>ESEKIYKVMEEIFVDRHYKENIRTGEEVKQYFSKSKAEFILRWSSANESDTENKYVFIAASFQASDGIHSIR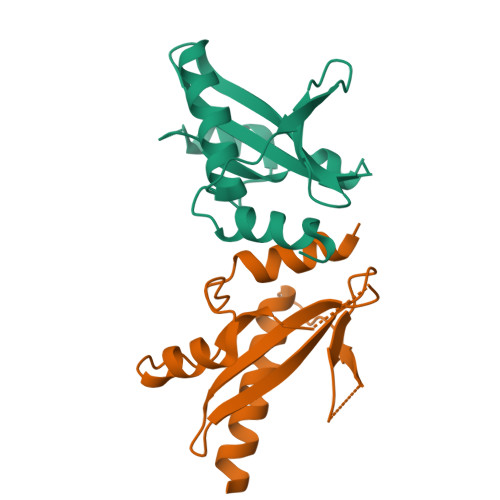YGINKNGELFSINTASNKVTPIDILPLGVMATLTQHITQNKELIEKAL[2x]> FQSNMHLPPLEPPISDRYFASGEVTIAADVVIAPGVLLIAEADSRIEIASGVCIGLGSVIHARGGAIIIQAGALLAAGVLIVGQSIVGRQACLGASTTLVNTSIEAGGVTAP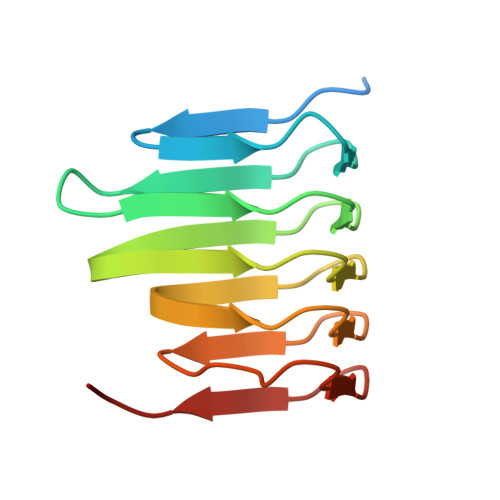GSLLSAETPP>SSMPLCPIDEAIDKKIKQDFNSLFPNAIKNIGLNCWTVSSRGKLASCPEGTAVLSCSCGSACGSW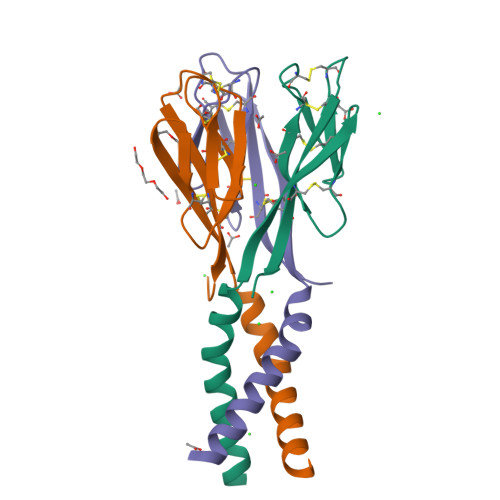DIREEKVCHCQCARIDWTAARCCKLQVAS[3x]(2S)-1-[4-[[(3S)-1,1-bis(oxidanylidene)thiolan-3-yl]methyl-methyl-amino]-6-methyl-pyrimidin-2-yl]-N-methyl-pyrrolidine-2-carboxamide 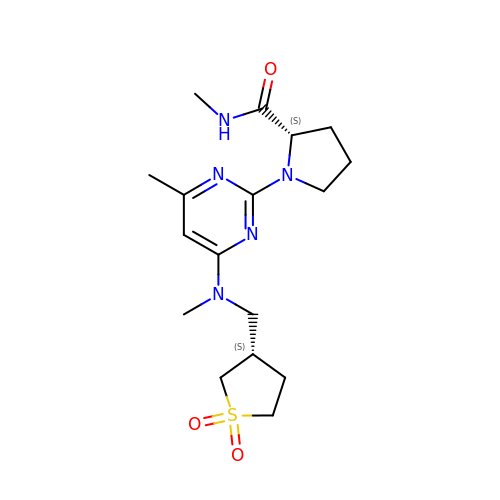| C17 H27 N5 O3 S | FPDVOQXTUVFQHW-KBPBESRZSA-N In prokaryotic organisms, several ubi gene clusters encoding a set of enzymes (UbiA, UbiB, UbiC, UbiD, UbiE, UbiF, UbiG, UbiH, and UbiX) produce ubiquinone from its precursor, chorismate. The monomer structure adopts a typical Rossmann-fold topology comprising eight α-helices (residues 19–32, 42–52, 60–71, 89–91, 107–115, 121–132, 147–159, and 177–192) and six β-strands (residues 8–13, 35–40, 78–81, 99–103, 135–140, and 162–165). The crystallographic symmetries of both crystal structures generate spherical dodecamers with dimensions of 105 Å × 93 Å × 95 Å. The monomeric structure of CpsUbiX is stabilized by two different patches of inter-subunit contacts, namely patches 1 and 2, to generate a dodecamer.

FMN-bound CpsUbiX crystallized in the orthorhombic space group (C2221) with 6 monomers in the asymmetric unit, while FMN-free CpsUbiX crystallized in the cubic space group (P23) with one molecule in the asymmetric unit. Electron density for FMN could be seen clearly in the subunit interface region of the complex crystal structure. FMN is bound to a positively charged groove in the subunit interface formed by three neighboring protomers. The FMN-binding site is surrounded by the α2 and α6 helices and the C-terminal loop region from another subunits. The phosphoribityl group of FMN is buried deeply in the groove, whereas the isoalloxazine ring remains partially accessible to the solvent. The C-terminal residue, Tyr204, forms a stacking interaction with FMN. In addition, the hydrophobic residues, Val47, Ile46, Trp86, and Tyr171 delimit the hydrophobic part of the isoalloxazine moiety of FMN. The phosphate group of FMN forms three hydrogen bonds with Ser41, Ser106, and Thr109. In contrast to FMN-free CpsUbiX, the FMN-bound CpsUbiX possesses a sharp turn at Ile198, causing the C-terminal end to point toward the interface between neighboring monomers, where FMN is bound. The charged surface is more prominent in FMN-bound CpsUbiX.

>GSHMNNDFNGKITLAITGASGASYAMRLIECLIAANYQLYILCSSAGRIVLDTEVGVKIPSSPDAASKFLTEKYQAKDQQITVFGKEQWFSPVASGSSAPKQMVVCPCSTGTMAAICHGMSDNLIERAADVVIKERGQLILMVRETPFSTLHLQNMLSLSQQGVTIMPASPGFYHKVETIEDLIDFMVGRVLDHLGIEQDIMPRWGYNI[6x]> SNANYMETGDQRFGDLVFRQLAPNVWQHTSYLDMPGFGAVASNGLIVRDGGRVLVVDTAWTDDQTAQILNWIKQEINLPVALAVVTHAHQDKMGGMDALHAAGIATYANALSNQLAPQEGMVAAQHSLTFAANGWVEPATAPNFGPLKVFYPGPGHTSDNITVGIDGTDIAFGGCLIKDSKAKSLGNLGDADTEHYAASARAFGAAFPKASMIVMSHSAPDSRAAITHTARMADKLR

NDM-1 has been reported to be a highly potent carbapenem-hydrolyzing, zinc-dependent MBL. NDM-1 is an extended spectrum zinc dependent β-lactamase capable of hydrolyzing nearly all classes of β-lactams, impairing the ability to treat life-threatening infections with intravenously and orally available carbapenems.. NDM-1 resembles the common β-lactamase fold, although it shows low sequence similarity to β-lactamases deposited in PDB (20–33% sequence identity). Our results show that NDM-1 is unique among other MBLs due to its enlarged and flexible active site, and explain the observed extended spectrum β-lactamase activity.

Three of our apoNDM-1 structures are zinc-free and are the first structures of a wild-type apo-enzyme in subclass B1. The three apoNDM-1 structures include two pairs of monomers A and B and one monomer A, and the structure of monometalated NDM-1 (mZnNDM-1 Δ36NY) includes four monomers (A, B, C, D), respectively in the asymmetric unit, providing nine crystallographically independent views of the molecule for NDM-1 Δ38, NDM-1 Δ36NY (monoclinic), NDM-1 Δ36NY (orthorhombic), mZn-NDM-1 Δ36NY (tetragonal). In our three apo and one monozinc structures, there are nine independent representations of NDM-1 molecules with different crystallization conditions and packing environments. In these structures, most active site loops show very small conformational changes with the exception of ASL1 and to some extent ASL4. These are key loops contributing to the expansion of active site accessibility. ASL1 shows the ability of assuming several alternative conformations that may be important for binding ligands. The structure of zinc-free NDM-1, along with the previously reported structures, provides important insight into the conformational changes associated with the metal binding properties of NDM-1.> DHNPFISVEWLKGPILEATAGDELVKLPVKLAAYPPPEFQWYKDGKALSGRHSPHALVLKEVTEASTGTYTLALWNSAAGLRRNISLELVVNVPPQIHEKEASSPSIYSRHSRQALTCTAYGVPLPLSIQWHWRPWTPCKM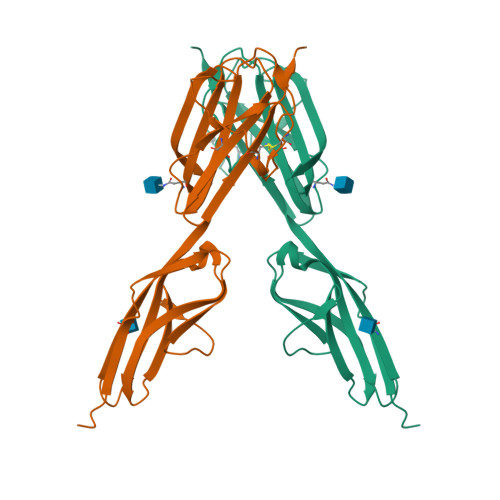FAQRSLRRRQQQDLMPQCRDWRAVTTQDAVNPIESLDTWTEFVEGKNKTVSKLVIQNANVSAMYKCVVSNKVGQDERLIYFYVTTHHHHHH>[2x]CAPSYQINS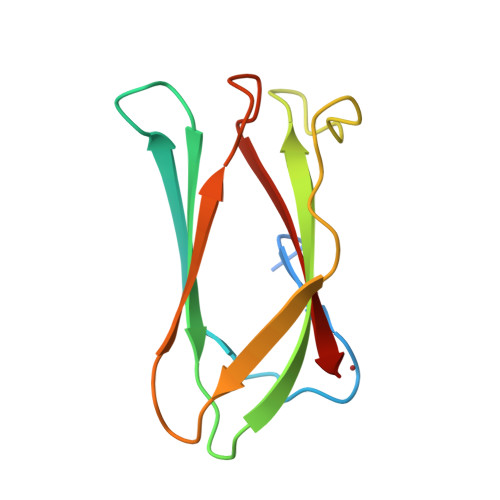NQNTVILGSNLPKSLVKQFQKRINSNGYLEFEVILRSTFAKDVIYKVDWLDKDGFVLRDVLNEDYQALRIPAGQEVILRKLASDTRANDFRLEIKAKN4-[2-AMINO-5-(2,3-DIHYDROTHIENO[3,4-B][1,4]DIOXIN-5-YL)PYRIDIN-3-YL]BENZAMIDE | C18 H15 N3 O3 S | 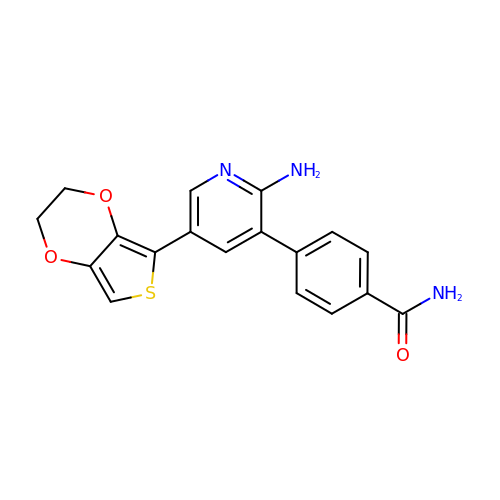AWUXFIAHZKNRJF-UHFFFAOYSA-N> MASDGVVVEIGKVTGSVGTTVEIPVYFRGVPSKGIANCDFVFRYDPNVLEIIGIDPGDIIVDPNPTKSFDTAIYPDRKIIVFLFAEDSGTGAYAITKDGVFAKIRATVKSSAPGYITFDEVGGFADNDLVEQKVSFIDGGVNVG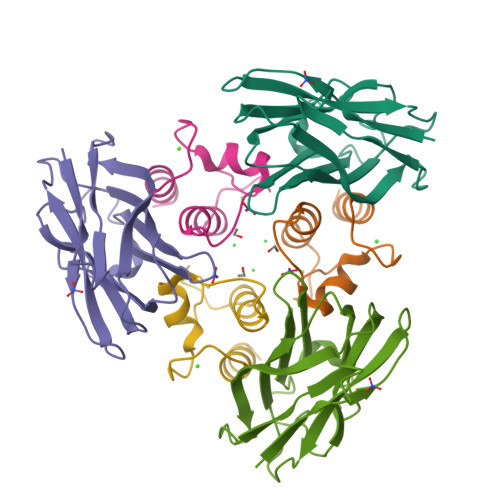NATPTKGATPTNTATPTK;> MGDVNGDGTINSTDLTMLKRSVLRAITLTDDAKARADVDKNGSINSTDVLLLSRYLLRVI>[8x]MPHRFKVYNYMSPTFC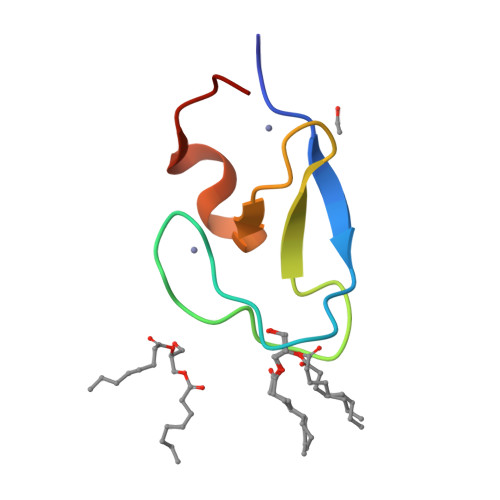DHCGSLLWGLVKQGLKCEDCGMNVHHKCREKVANLCG3-[3-(4-methoxyphenyl)-2-(1H-thieno[3,2-c]pyrazol-3-yl)-1H-indol-6-yl]pentan-3-ol 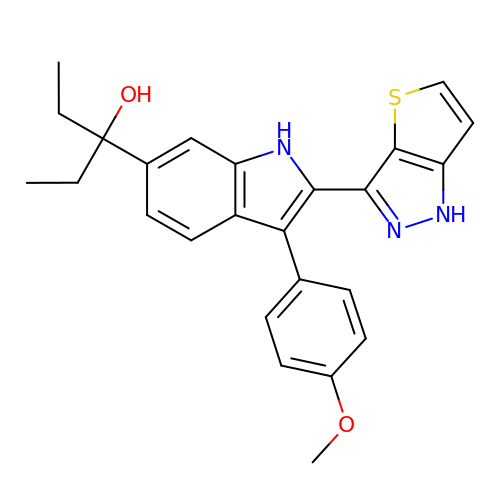| C25 H25 N3 O2 S | LXMWGYNOGUKODT-UHFFFAOYSA-N> MPETCPNTVTKRRCAVVTGGNKGIGFEICKQLSSNGIMVVLTCRDVTKGHEAVEKLKNSNHENVVFHQLDVTDPIATMSSLADFIKTHFGKLDILVNNAGVAGFS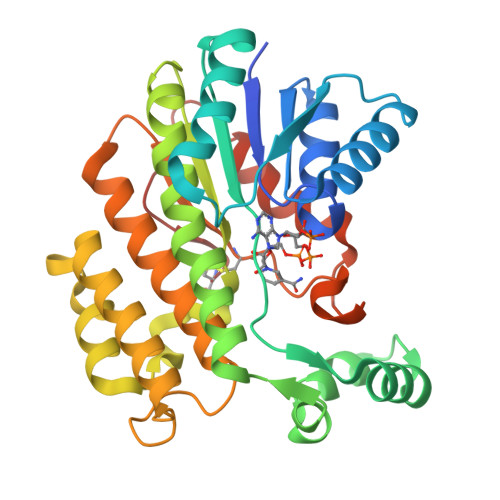VDADRFKAMISDIGEDSEELVKIYEKPEAQELMSETYELAEECLKINYNGVKSVTEVLIPLLQLSDSPRIVNVSSSTGSLKYVSNETALEILGDGDALTEERIDMVVNMLLKDFKENLIETNGWPSFGAAYTTSKACLNAYTRVLANKIPKFQVNCVCPGLVKTEMNYGIGNYTAEEGAEHVVRIALFPDDGPSGFFYDCSELSAF>[2x]MANEEDDPVVQEIDVYLAKSLAEKLYLFQYPVRPASMTYDDIPHLSAKIKPKQQKVELEMAIDTLNPNYCRSKGEQIALNVDGACADETSTYSSKLMDKQTFCSSQTTSNTSRYAAALYRQGELHLTPLHGILQLRPSFSYLDKADAKHREREAANEAGDSSQDEAEDDVKQITVRFSRPESEQARQRRVQSYEFLQKKHAEEPWVHLHYYGLRDSRSEHERQYLLCPGSSGVENTELVKSPSEYLMMLMPPSQEEEKDKPVAPSNVLSMAQLRTLPLADQIKILMKNVKVMPFANLMSLLGPSIDSVAVLRGIQKVAMLVQGNWVVKSDILYPKDSSSPHSGVPAEVLCRGRDFVMWKFTQSRWVVRKEVATVTKLCAEDVKDFLEHMAVVRINKGWEFILPYDGEFIKKHPDVVQRQHMLWTGIQAKLEKVYNLVKETMPKKPDAQSGPAGLVCGDQRIQVAKTKAQQNHALLERELQRRKEQLRVPAVPPGVRIKEEPVSEEGEEDEEQEAEEEPMDTSPSGLHSKLANGLPLGRAAGTDSFNGHPPQGCAPTPVARELKAFVEATFQRQFVLTLSELKRLFNLHLASLPPGHTLFSGISDRMLQDTVLAAGCKQILVPFPPQTAASPDEQKVFALWESGDMSDQHRQVLLEIFSKNYRVRRNMIQSRLTQECGEDLSKQEVDKVLKDCCVSYGGMWYLKGTVQS

Pol III is a multi-subunit complex composed of 17 subunits. The TFIIF-like RPC4/5 and the TFIIE-like RPC3/6/7 subcomplexes are Pol III specific and can be regarded as built-in general transcription factors that play a fundamental role in Pol III transcription initiation and termination. A notable exception is the subunit RPC5, which in metazoans encompasses a long C-terminal extension (RPC5EXT, ~450 residues long), whose function is currently unknown. The RPC5EXT is formed by two consecutive tandem winged helix domains (tWHD1 residues 259–440; tWHD2 residues 556–708) connected by a 115 residue-long flexible linker.

To gain insight into the structure and function of RPC5EXT, we determined the structure of its individual domains by X-ray crystallography. Of the two tWHDs, tWHD1 is the most conserved while tWHD2 is absent in Caenorhabditis elegans and Drosophila melanogaster. The tWHD2 structure revealed a dimer formed by domain swapping. This arrangement is likely caused by the crystallization conditions and, in agreement with this hypothesis, SAXS data showed a monomeric conformation as the most likely in solution. Nevertheless, the two possible conformations of tWHD2, compact or elongated, suggests a degree of flexibility within this domain. Thus, one possibility is that, analogously to A49 tWHD, the RPC5-tWHD1 participates in an interaction with the upstream DNA and bound transcription factors, thus stabilizing the human Pol III PIC. In addition, the Dali server analysis retrieved similarities between the individual WHDs of RPC5EXT tWHD2 and the WHDs of cullin and cullin-like proteins, which are involved in ubiquitin-dependent proteolysis. On the contrary, RPC5ΔtWHD2 and RPC5ΔC were rapidly degraded with RPC5ΔC almost completely depleted after only 2 h following cycloheximide treatment. Several abundant phosphorylation sites have been identified in RPC5EXT, which, together with the evidence of structural similarities between RPC5EXT tWHD2 and factors involved in targeted degradation, suggests the intriguing hypothesis of an RPC5EXT-mediated layer of regulation impacting overall Pol III abundance in response to environmental cues that may have evolved in higher organisms.>MDFECQFVCELKELAPVPALLIRTQTTMSELGSLFEAGYHDILQLLAGQGKSPSGPPFARYFGMSAGTFEVEFGFPVEGGVEGSGRVVTGLTPSGKAASSLYIGPYGEIEAVYDALMKWVDDNGFDLSGEAYEIYLDAPAETAPDQLRTRVSLML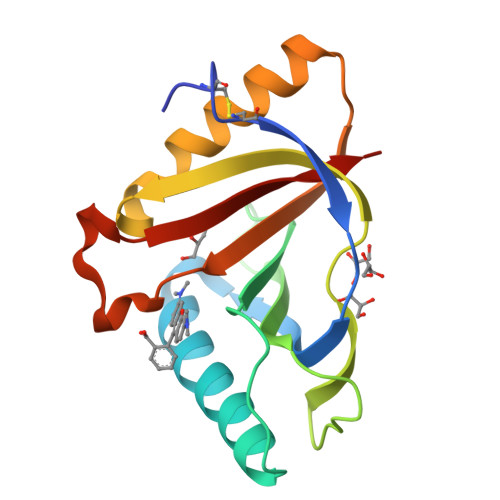HESLE[2x]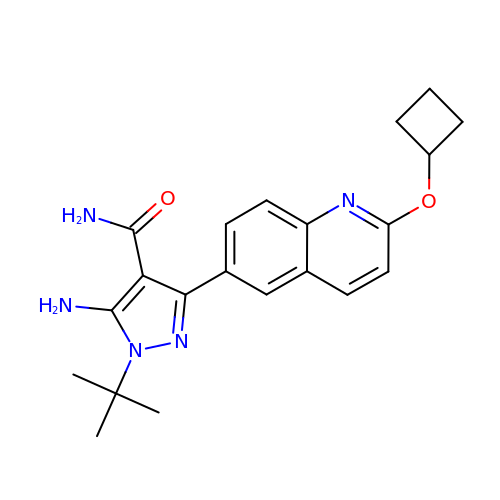5-amino-1-tert-butyl-3-[2-(cyclobutyloxy)quinolin-6-yl]-1H-pyrazole-4-carboxamide | C21 H25 N5 O2 | BTTULLMSRICKGC-UHFFFAOYSA-N> MVRSFIYEPFQIPSGSMMPTLLIGDFILVEKFAYGIKDPIYQKTLIETGHPKRGDIVVFKYPEDPKLDYIKRAVGLPGDKVTYDPVSKELTIQPGCSSGQACENALPVTYSNVEPSDFVQTFSRRNGGEATSGFFEVPKNETKENGIRLSERKETLGDVTHRILTVPIAQDQVGMYYQQPGQQLATWIVPPGQYFMMGDNRDNSADSRYWGFVPE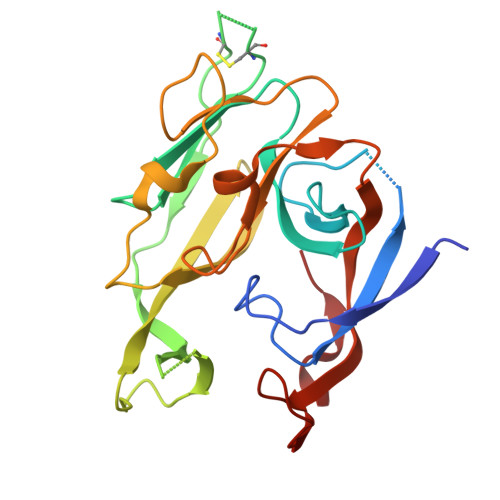ANLVGRATAIWMSFDKQEGEWPTGLRLSRIGGIH Echovirus 18 (E18), as a member of enterovirus species B, is a significant causative agent of aseptic meningitis and viral encephalitis in children. Echoviruses belong to enterovirus species B (EV-B) of the Enterovirus genus within the Picornaviridae family, which are single-stranded, positive RNA viruses (~30 nm) without a lipid envelope (nonenveloped virus). We describe the mechanism for the entry of certain EV-B serotypes by using FcRn as a two-in-one attachment-and-uncoating receptor. Protomers consist of the capsid protein (VP1, VP2, and VP3) and the smaller internal protein VP4.

E18 (strain HeB15-254) was purified by sucrose density centrifugation, and the fractions of mature virus particles were collected. Detailed characterizations of mature E18 particles, the E18/FcRn complex under physiological conditions (pH 7.4), and the E18/FcRn complex under acidic conditions (pH 5.5) were performed. The density map of all three particles showed clear protein backbones and side chains of most residues, which allowed us to build the atomic model. The E18 mature particle has a pseudo-T=3 symmetry arrangement resembling other picornavirus architectures. Sixty copies of the protomer-packaged mature particles had a diameter of 30 nm. The mature E18 particles alone did not exhibit significant changes under acidic conditions.

> GDNQDRTVANTQPSGPSNSKEIPALTAVETGHTSQVDPSDTLQTRHVVNFHSRSESTVENFMGRAACVFMDQYKLNGEETSTDNFAVWTINVREMAQLRRKCELFTYMRFDIEMTMVITSCQDQGTQLEQDMPVLTHQIMYVPPGGPIPAKVDSYEWQTSTNPSVFWTEGNAPARMSIPFISVGNAYSLFYDGWSHFTQDGTYGYTTLNAMGKLFVRHVNKSSPHQITSTIRVYFKPKHIKAWVPRPPRLCPYINKGDVNFVVTEVTDARKSITDTP;> SPSAEECGYSDRVRSMTLGNSTITTQESANVVVGYGEWPSYLSDKEATAEDQPTQPDVATCRFYTLESVQWEKSSPGWWWKFPEALKNMGLFGQNMHYHYLGRAGYTIHVQCNASKFHQGCLLVVCVPEAEMGCADTSTTFPATELTTEEEPHVFTSDSITGKKVQAAVCNAGMGVGVGNLTIFPHQWINLRTNNSATIVMPYINSVPMDNMFRHYNFTLMIIPFAPLNFNEGATAYVPVTVTIAPMYAEYNGLRLASTQ;> GVPVLNTPGSTQFLTSDDFQSPSAMPQFDETPEMHIPGEVRNLMEMAEVDSVVPVNNITGKTKSMEAYQIAVGTGNTDKTKPIFSFQMDPGYSSVLKRTLLGEMLNYYAHWSGSVKLTFLFCGSAMATGKLLISYSPPGASVPSSRKDAMLGTHIIWDIGLQSSCVLCVPWISQSHYRMVQQDPYTSAGYITCWYQTNIVVPPGAPTSCDVLCFASACNDFSVRLLRDTPFMAQPGKLQ;> MGAQVSTQKTGAHETSLNAKGNSIIHYTNINFYKDAASSASNRQELQQDPGKFTDPVKDLMVKTLPALN> MDLLKRHLAPIVPDAWSAIDEEAKEIFQGHLAGRKLVDFRGPFGWEYAAVNTGELRPIDDTPEDVDMKLRQVQPLAEVRVPFTLDVTELDSVARGATNPDLDDVARAAERMVEAEDSAIFHGWAQAGIKGIVDSTPHEALAVASVSDFPRAVLSAADTLRKAGVTGPYALVLGPKAYDDLFAATQDGYPVAKQVQRLVVDGPLVRANALAGALVMSMRGGDYELTVGQDLSIGYAFHDRSKVELFVAESFTFRVLEPGAAVHLRYA

Encapsulins are protein nanocompartments that house various cargo enzymes, including a family of decameric ferritin-like proteins. Cargo enzymes are directed inside the encapsulin nanocompartment by a terminal localization sequence (LS) that binds to the interior face of the encapsulin. EncFtn oxidizes iron in a similar manner to other ferritins, but due to its open structure, it must be associated with an encapsulin nanocage to act as an iron store. Together, the encapsulin EncFtn (Enc:EncFtn) complex can perform both the oxidation and storage functions of classical ferritins. Here, we investigate the structure of the Enc:EncFtn nanocompartment from the halophilic bacterium Haliangium ochraceum to gain a better understanding of the arrangement and stoichiometry of the complex.

Motivated by the apparent interior density in the Loaded-Enc sample, we performed single-particle cryo-EM on the Loaded-Enc nanocompartment complex. The reconstruction displays a T = 1 icosahedral arrangement of 60 encapsulin monomers, with clearly resolved secondary structure elements. Small pores are visible in the shell at, or close to, the two-, three-, and fivefold symmetry axes, where protein monomers interact with each other. Regions of the reconstruction around the icosahedral fivefold axes displayed a lower resolution than the other regions of the structure in a local resolution map. The monomer of the encapsulin nanocompartment from the reconstruction displays a HK97-fold typical for encapsulins, with the position of the E-loop broadly determining the topology of the encapsulin nanocage. With the imposition of I1 symmetry on the reconstruction, the EncFtn cargo is not visible within the lumen. This suggests that the organization of the EncFtn protein within the encapsulin shell does not conform to icosahedral symmetry and is rotationally averaged through our symmetry-imposed processing.>[2x]AEAGITGTWYNQLGSTFIVTAGADGALTGTYESAVGNAESRYVLTGRYDSAPATDGSGTALGWTVAWKNN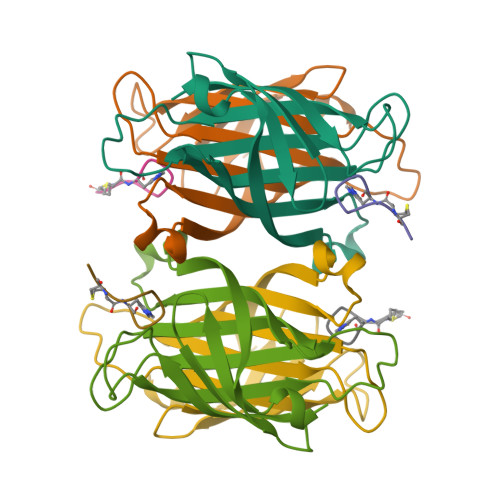YRNAHSATTWSGQYVGGAEARINTQWLLTSGTTEANAWKSTLVGHDTFTKVKP;>HPQGPPCKX[2x]>[2x]GFKQDIATIRGDLRTYAQDIFLAFLNKYPDERRYFKNYVGKSDQELKSMAKFGDHTEKVFNLMMEVADRATDCVPLASDAN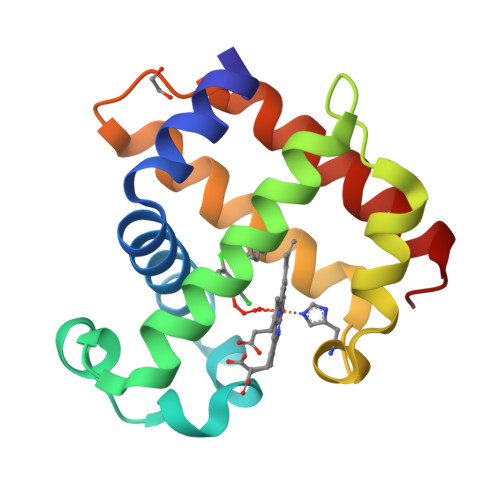TLVQMKQHSSLTTGNFEKFFVALVEYMRASGQSFDSQSWDRFGKNLVSALSSAGMK>[4x]SNAMSLEKLDTNTFEQLIYDEGK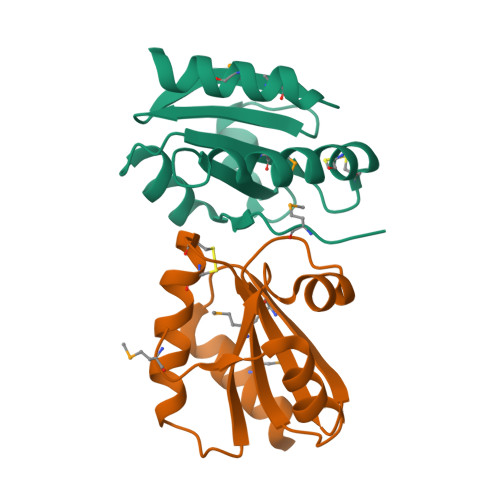ACLVMFSRKNCHVCQKVTPVLEELRLNYEESFGFYYVDVEEEKTLFQRFSLKGVPQILYFKDGEYKGKMAGDVEDDEVEQMIADVLED> EVVLLDFAAAGGELGWLTHPYGKGW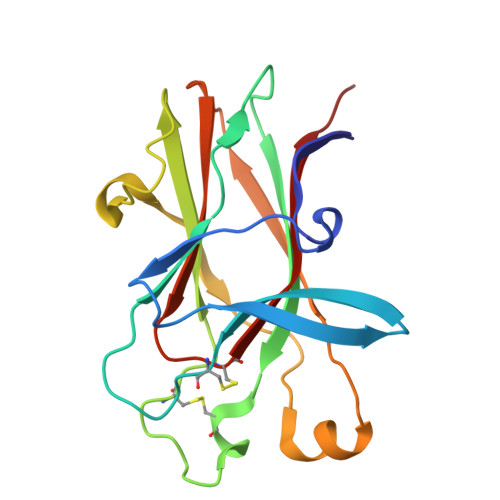DLMQNIMNDMPIYMYSVCNVMSGDQDNWLRTNWVYRGEAERIFIELKFTVRDCNSFPGGASSCKETFNLYYAESDLDYGTNFQKRLFTKIDTIAPDEITVSSDFEARHVKLNVEERSVGPLTRKGFYLAFQDIGACVALLSVRVYYKKC>[2x]MDRVGKYGLFIKRISPKDADITKESLETVNNMLVFLAEKLTKQANIIIDQKTLRHDAFLWLLTDIQGELGKHSQDFANSVLYGEKELVFPTKRTENLMRKNTCLRISQSAVKTLTAILEYFCGQIMEASFSQAKKSKRKRIRPIDIEAAISQDKELHSMFGKGVISGR;>[2x]MSKAG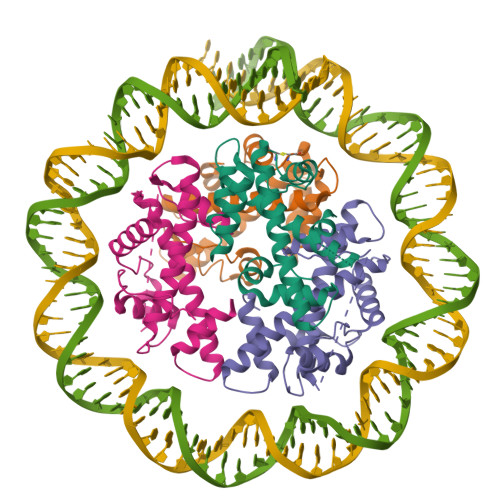KKVKAQQHGHLADHVSVGETQIPKASTQHLLRKAGSLSAAGDTEVPIRGFVHMKLHKLVQKSLLAMQLAKRKTIMKSDVKKAAELMHLPVFAIPTKDSGAKGSVFLSCRQKGAGSAGTGSETNSQEVRSQMKSTCLIIPKERFRTMAKEISKKEGHDVHIAEAALDMLQVIVESCTVRLLEKALVITYSGKRTRVTSKDIETAFMLEHGPL>NNILFGLSHEGSHPQTLHAAQSLELSSFRFTMQSDCNLVLFDSDVRVWASNTAGATGCRAVLQSDGLLVILTAQNTIRWSSGTKGSIGNYVLVLQPDRTVTIYGPGLWDSGTSNKGSVVVANNGNSILYSTQGNDNHPQTLHATQSLQLSPYRLSMETDCNLVLFDRDDRVWSTNTAGKGTGCRAVLQPNGRMDVLTNQNIA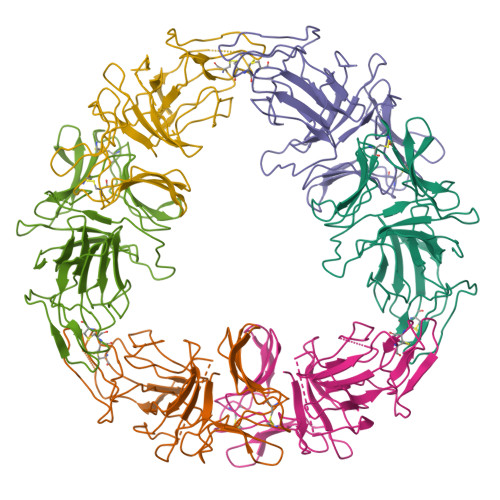VWTSGNSRSAGRYVFVLQPDRNLAIYGGALWTTG[6x]ICV, however, has only one major surface glycoprotein, the hemagglutinin-esterase-fusion (HEF) protein, which possesses all-in-one of receptor binding, receptor destroying and membrane fusion activities. To further evaluate the infectivity and transmissibility of IDV, we expressed and purified the ectodomain of D/OK HEF, and determined that it also uses 9-O-Acetyl-Sia as its receptor by glycan microarray. We also solved the crystal structure of D/OK HEF, both in its native state (resolution of 2.4 Å) and in complex with its receptor analogue (resolution of 3.1 Å), and the structure of the enzymatically inactive HEF (resolution of 2.4 Å) alone and in complex with two receptor analogs respectively (both resolutions of 2.2 Å). Indeed, our results show that IDV HEF is functionally and structurally similar to ICV HEF, but with some distinct characteristics.

To avoid the enzymatic cleavage of the receptor substrates, we generated the catalytic mutant for the binding experiments and for the structures of the relevant complexes. Thus, we designed the enzymatically inactive HEF protein (HEF-mut) containing S57A, D356A and H359A substitutions, and expressed it using the same method as wild type protein. For the IDV HEF-mut/receptor complex structures, interpretable electron density is observed for all the three glycan rings of 9-O-Ac-3'SleC, including Neu5,9Ac2 (9-O-Ac-Sia-1), galactose-2 (Gal-2), and N-acetylglucosamine-3 (GlcNAc-3); while for 9-O-Ac-3'SLN, electron density for the first two sugars is well defined. The glycan rings of 9-O-Ac-3'SleC go through the open channel between the 230-helix and 270-loop. The open channel in the receptor-binding cavity of IDV could provide a structural basis for accommodating different receptors with diverse glycan rings in different cell types, which should be tested in the future. But the majority of the interactions between ligands and IDV HEF are made by the 9-O-Ac-Sia-1 moiety, whereas the glycan portion of the ligands do not make significant contacts with IDV HEF, except for a hydrogen bond between the Gal-2 of 9-O-Ac-3'SLN and S173. Compared with the ICV HEF receptor complex, the 9-O-Ac-Sia-1 of the receptor bound to IDV HEF displays a very similar orientation. The 9-O-acetyl group of the receptor docks into a nonpolar, hydrophobic pocket, formed by V275, F229, F240 and F297. The absence of two hydrogen-bonding interactions between hydroxyl group of Y127 and the 8-hydroxyl and 9-amide of the ligand, pushes the 9-O-acetyl moiety of 9-O-Ac-sia-1 to the other side by ~1.1 Å.

>[2x]ELICIVQRVNESFSLHSGFGGNVYSMKTEPMTGFTNVTKGASVINQKDWIGFGDARTDLTNDQFPASSDVPLAVAKKFRSLSGASLMLSAFGPPGKVDYLYQGCGKEKVFYEGVNWSPEAGIDCFGSNWTQTKKDFYSRIYEAARSSTCMTLVNSLDTKISSTTATAGTASSCSSSWMKSPLWYAESSVNPGAKPQVCGTEQSATFTLPTSFGIYKCNKHVVQLCYFVYENKAKFNTFGCGDYYQNYYDGNGNLIGGMDNRVAAYRGIANAGVKIECPSKILNPGTYSIKSTPRFLLVPKRSYCFDTDGGYPIQVVQSEWSASRRSDNATEEACLQTEGCIFIKKTTPYVGEAADNAGDIEMRQLLSGLGNNDTVCVSQSGYTKGETPFVKDYLSPPKYGRCQLKTDSGRIPTLPSGLIIPQAGTDS;>FGLLFVGFVAGGVAGGYFWGRSNGGGGGASVSSTQAGFDKIGKDIQQLRNDTNAAIEGFNGRIAHDEQAIKNLAKEIEDARAEALVGELGIIRSLIVANISMNLKESLYELANQITKRGGGIAQEAGPGCWYVDSENCDASCKEYIFNF[2x]> GSGQDIQL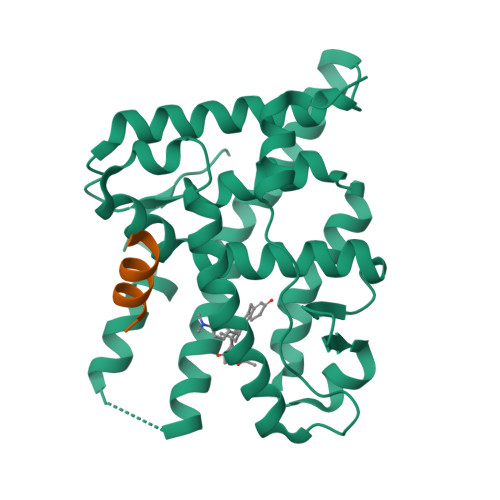IPPLINLLMSIEPDVIYAGHDNTKPDTSSSLLTSLNQLGERQLLSVVKWSKSLPGFRNLHIDDQITLIQYSWMSLMVFGLGWRSYKHVSGQMLYFAPDLILNEQRMKESSFYSLCLTMWQIPQEFVKLQVSQEEFLCMKVLLLLNTIPLEGLRSQTQFEEMRSSYIRELIKAIGLRQKGVVSSSQRFYQLTKLLDNLHDLVKQLHLYCLNTFIQSRALSVEFPEMMSEVIAAQLPKILAGMVKPLLFHKK;> TNMGLEAIIRKALMGKY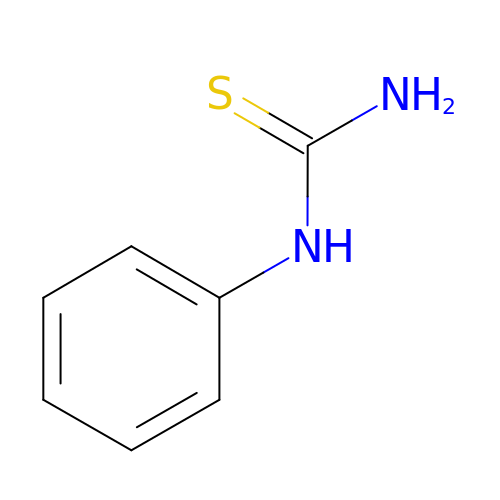N-PHENYLTHIOUREA | C7 H8 N2 S | FULZLIGZKMKICU-UHFFFAOYSA-N>QELGNANFENFIGATEGFSEIAYQFTSHILTLGYAVMLAGLLYFILTIKNVDKKFQMSNILSAVVMVSAFLLLYAQAQNWTSSFTFNEEVGRYFLDPSGDLFNNGYRYLNWLINVPMLLFQILFVVSLTTSKFSSVRNQFWFSGAMMIITGYIGQFYEVSNLTAFLVWGAISSAFFFHILWVMKKVINEGKEGISPAGQKILSNIWILFLISWTLYPGAYLMPYLTGVDGFLYSEDGVMARQLVYTIADVSSKVIYGVLLGNLAITLSKNKEL[5x]

Microbial rhodopsins (MRs) are transmembrane light-sensitive proteins, found in Archaea, Bacteria, Eukaryota, and also viruses. MRs are composed of seven transmembrane α-helices (A–G) with the cofactor retinal covalently bound to the lysine residue of helix G via the Schiff base (RSB). Despite this paradigm, the first light-driven Na+ pump KR2 was identified in Krokinobacter eikastus in 20132. KR2 contains a characteristic for all known Na+-pumping rhodopsins (NaRs) set of N112, D116, Q123 residues in the helix C (NDQ motif).

To understand better the nature of conformational switches in KR2 and the influence of D116 protonation on the protein conformation, we produced and crystallized KR2-D116N at pH 8.0, which mimics the WT protein with fully protonated D116 and solved its structure in the pentameric form at 2.35 Å. Confirming our hypothesis, the structure shows that introduction of asparagine at the position of D116 led to the flip of the side chains of N112 and L74 in comparison to the ground state of the wild type (WT) protein and disappearance of the SBC1, characteristic for the ‘expanded’ conformation. Overall, the structure of D116N is very similar to that of the O-state (RMSD 0.2 Å) and also to the ‘compact’ conformation (RMSD 0.3 Å) of the KR2-WT. However, Na+ is absent inside the protomers and the relative orientation of the RSBH+ and N116 is altered. Particularly, the RSBH+ forms two alternative conformations, and hydrogen bond between the RSBH+ and N116 is absent.We also observed that D116 protonation destabilizes the pentameric assembly of KR2. Thus, we suggest that neutralization of D116 is the key determinant of the formation of the ‘compact’ conformation, which explains their structural similarity. Importantly, the organization of the pIRC2 region is identical in the O-state and KR2-D116N. It means that the rearrangements on the surface of the KR2 occur not directly in response to the retinal isomerization upon photon absorption, but rather due to the redistribution of charges in the central inner part of the protein protomer.> GAMGSGMAMDTFITRNFQTTIIQK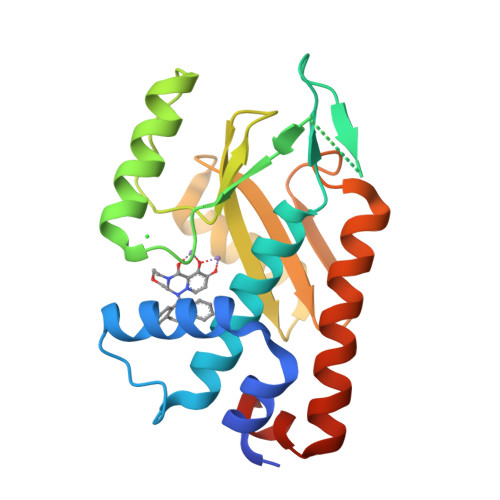AKNTMAEFSEDPELQPAMLFNTCVHLEVCYVISDMNFLDEEGKSYTALEGQGKEQNLRPQYEVIEGMPRTIAWMVQRSLAQEHGIETPKYLADLFDYKTKRFIEVGITKGLADDYFWKKKEKLGNSMELMIFSYNQDYSLSNESSLDEEGKGRVLSRLTELQAELSLKNLWQVLIGEEDVE[(1S)-1-FLUORO-2-(HYDROXYAMINO)-2-OXOETHYL]PHOSPHONIC ACID | C2 H5 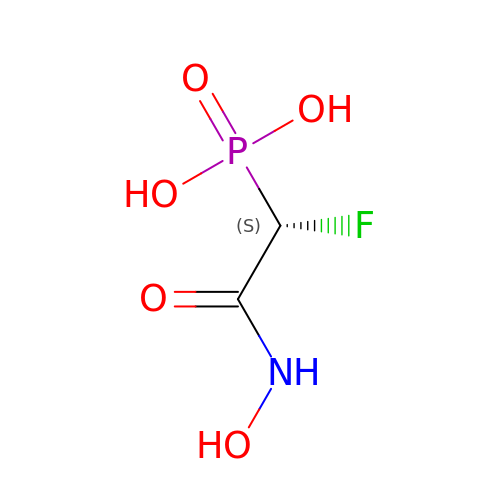F N O5 P | PDPXHRBRYUQCQA-SFOWXEAESA-N>[2x]GSLSKVEESQLNEKENKNVADGLAWSYYFGYLKFVLPELEKQIEKTSKFRSKEKFVKKMFILIPSNCFWDDKIPGSDYDPQNRITFEGNTEPLEKTRGGVFLRHYKHSV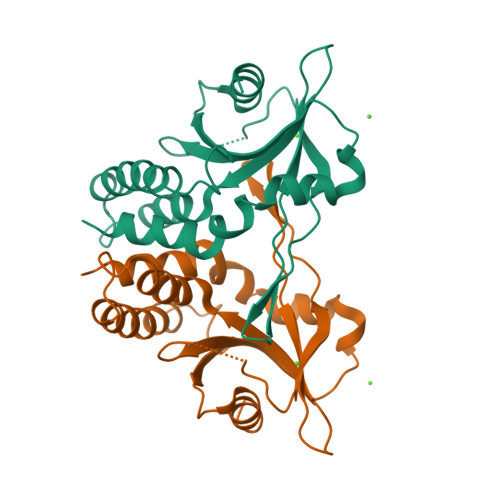YEIKDGENEPWFCIMEYATPLLTLYDMSVAQPGELSREERDAQVVVFLRKLQDILEGDRACQGKYELVTFSPDRDLADVMLRKLKDSELEIGG>[2x]GMSVVTSFYPMYAMTKEVSGDLNDVRMIQSGAGIHSFEPSVNDVAAIYDADLFVYHSHTLEAWARDLDPNLKKSKVNVFEASKPLTLDRVKPGATVYDPHTWTDPVLAGEEAVNIAKELGHLDPKHKDSYTKKAKAFKKEAEQLTEEYTQKFKK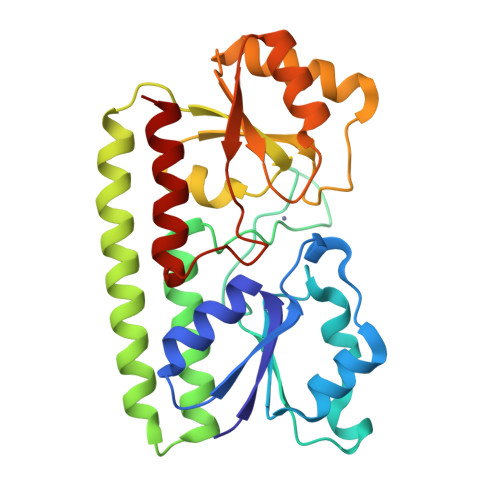VRSKTFVTQHTAFSYLAKRFGLKQLGISGISPEQEPSPRQLKEIQDFVKEYNVKTIFAEDNVNPKIAHAIAKSTGAKVKTLSPLEAAPSGNKTYLENLRANLEVLYQQLK>[2x]XPLVVAASII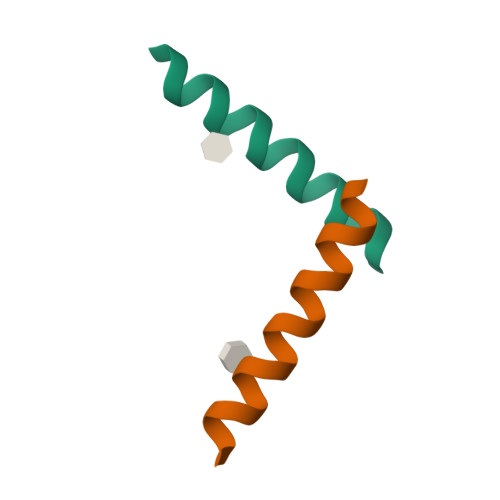AILHLILWELDRLX>[8x]AMAISDPQSSTRNELETGSSSACPKVIYIFARASTEPGNMGISAGPIVADALERIYGANDVWVQGVGGPYL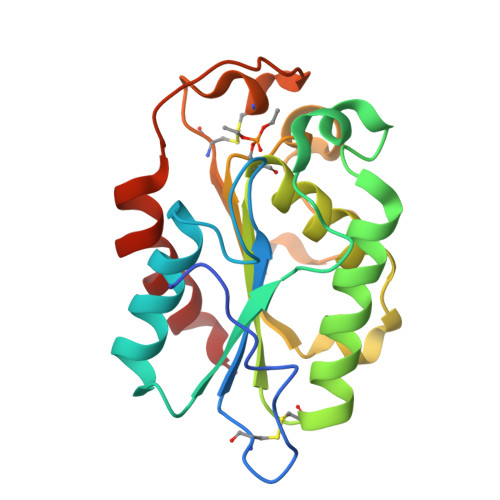ADLASNFLPDGTSSAAINEARRLFTLANTKCPNAAIVSGGYSQGTAVMAGSISGLSTTIKNQIKGVVLFGYTKNLQNLGRIPNFETSKTEVYCDIADAVCYGTLFILPAHFLYQTDAAVAAPRFLQARIG N6-cyclopentyladenosine | 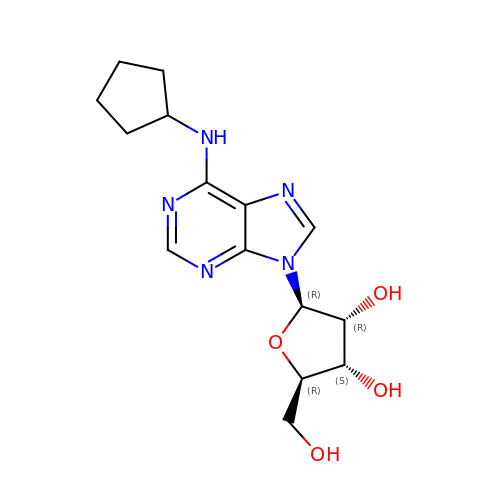C15 H21 N5 O4 | SQMWSBKSHWARHU-SDBHATRESA-N TETRADEC-13-YNOIC ACID - COA THIOESTER | C35 H58 N7 O17 P3 S | 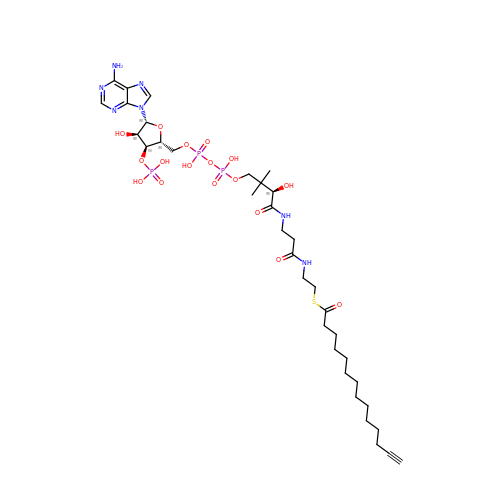YPDKCQHYDROOAS-QSGBVPJFSA-N>[2x]GRRRVTDERE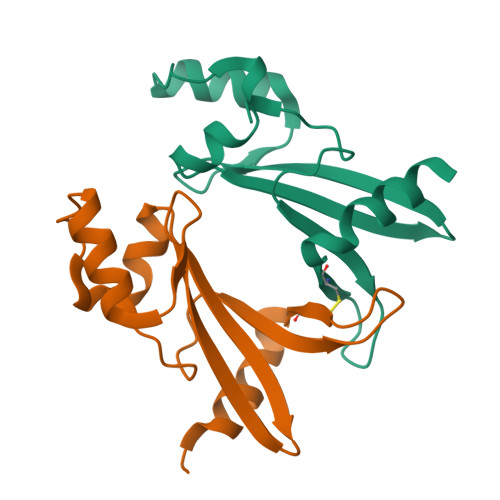LRIPLEYGWQRETRIRNFGGRLQGEVAYYAPCGKKLRQYPEVIKYLSRNGIMDISRDNFSFSAKIRVGDFYEARDGPQGMQWCLLKEEDVIPRIRAMEGRRG> MDAEEKMGVELSSPSAIMEHARRLYMSKDYRSLESLFGRCLKKSYNLDLWMLYIEYVRKVSQKKFKLYEVYEFTLGQFENYWDSYGLYKEYIEEEGKIEDEQTRIEKIRNGYMRALQTPMGSLSELWKDFENFELELNKITGKKIVGDTLPIFQSSFQRYQQIQPLIRGWSVKNAARLIDLEMENGMKLGGRPHESRMHFIHNYILDSFYYAEEVYFFYSEYLIGIGQKEKAKKVVERGIEMSDGMFLSLYYGLVMDEEAVYGDLKRKYSMGEAESAEKVFSKELDLLRINHLNYVLKKRGLELFRKLFIELGNEGVGPHVFIYCAFIEYYATGSRATPYNIFSSGLLKHPDSTLLKEEFFLFLLRIGDEENARALFKRLEKTSRMWDSMIEYEFMVGSMELFRELVDQKMDAIKADAILPPLPPREHNVQMEGILGRYHCFLDSFNFLDLKIR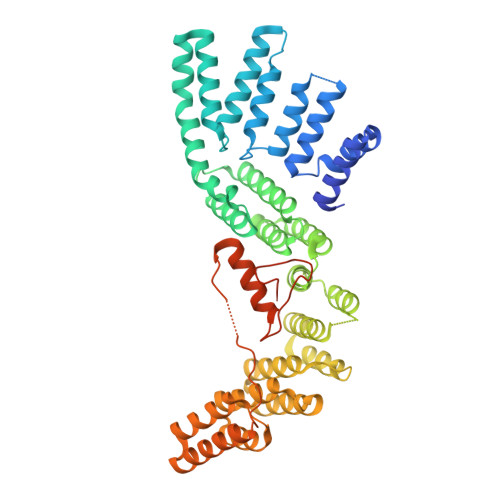DNSRLLDEFMENLPKISQQNNVLSNLRVEKVISLLKSVQ N-(benzylsulfonyl)-O-tert-butyl-D-seryl-N-(4-carbamimidoylbenzyl)glycinamide | C24 H33 N5 O5 S | 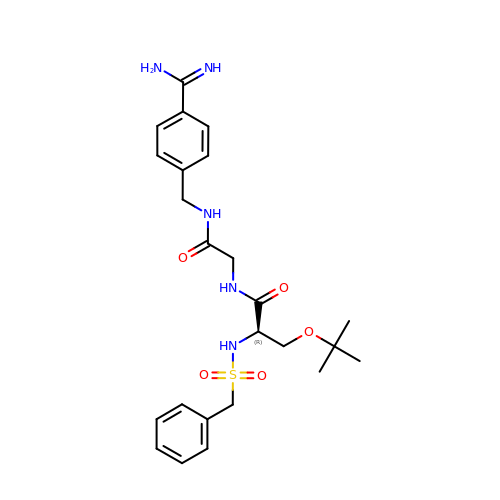NAEBSNBHOZLKPM-HXUWFJFHSA-N>[8x]MATKDLPTHLSSNTGFGKHHGKTQSHMAFENASTSVAASQMRNALNALAETVPDPNERKRFEAEMDNF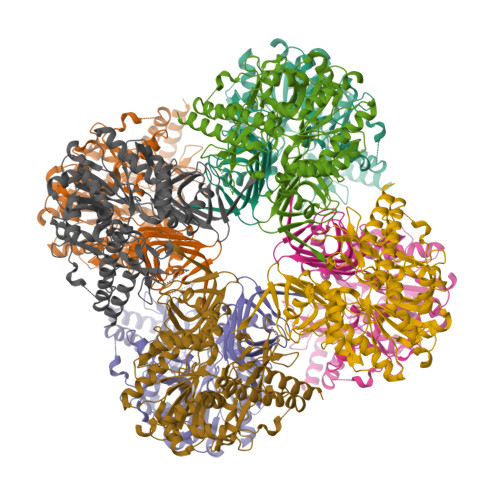FALFRRFLNDKAKGNVVNWDRIAPPQPSQVVNYDDIGKESSVEFLNKLAVVKLNGGLGTSMGCVGPKSVIEVREGMSFLDLSVRQIEHLNRTYNVNVPFVLMNSFNTDQDTQSIIKKYQGHNVDIITFNQSRYPRIIKDSLLPAPKSFDAPLQDWYPPGHGDVFESLYNSGTLDKLLERGVEYIFLSNADNLGAVVDTRILQHMIDTKAEYIMELTDKTKADVKGGTIIDYEGKVRLLEIAQVPKEHVNEFKSIKKFKYFNTNNIWMNLRAIKRVVEENELEMEIIANEKSIPADKKGEADQAIYQLETAVGAAIRHFKNAHGVNVPRRRFLPVKTCSDLLLVKSDLYRLEHGQLVMDPNRFGGVPVIKLGSDFKKVSDFQKRIPSIPRIVELDHLTITGAVNLGRNVTLKGTVIIVATEGSTIDIPPGSVLENCVVQGSLRILEH In this paper, the crystal structure of the complex of the DNA duplex d(AAAATTTT)2 with the dicationic drug 4,4′-bis(imidazolinylamino)diphenylamine (CD27) is presented. CD27 is chemically related to diamidines, a class of dicationic DNA minor-groove binders with a long history of clinical success as antiprotozoal agents. CD27, in particular, proved to be a potent inhibitor of Trypanosoma brucei growth in vitro and in vivo. The drug binds to the minor groove of DNA as expected, but it shows two new features that have not previously been described: (i) the drugs protrude from the DNA and interact with neighbouring molecules, so that they may act as cross-linking agents, and (ii) the drugs completely cover the whole minor groove of DNA and displace bound water.

The duplexes are stacked and organized as infinite continuous columns which cross in space at 60°. The drug molecules completely fill the minor groove of the DNA duplexes. No water molecules remain in the minor groove. Thus, the complex appears as a pseudo-continuous triple helix with one drug and two phosphodiester strands. Crossings are stabilized in part by the interaction of the drug molecules with neighbouring DNA phosphates. All three CD27 drugs form tight van der Waals interactions with the minor groove of DNA along the whole molecule. Drug D interacts with two phosphates, whereas drug E interacts with only one. Drug F has no external interactions. The duplexes are rather straight; the roll angles of individual steps have values of below 5°. An unexpected feature of the DNA structure is the high twist value in the AA/TT base steps, which have an average value of 38.5°.

>[3x]AAAATTTT>[2x]EKVDNPFEGAKLYVNPVWSAKAAAEPGGSAVANESTAVWLDRIGAIEGNDSPTTGSMGLRDHLEEAVRQSGGDPLTIQVVIYNLPGRDCAALASNGELGPDELDRYKSEYIDPIADIMWDFADYENLRIVAIIEIDSLPNLVTNVGGNGGTELCAYMKQNGGY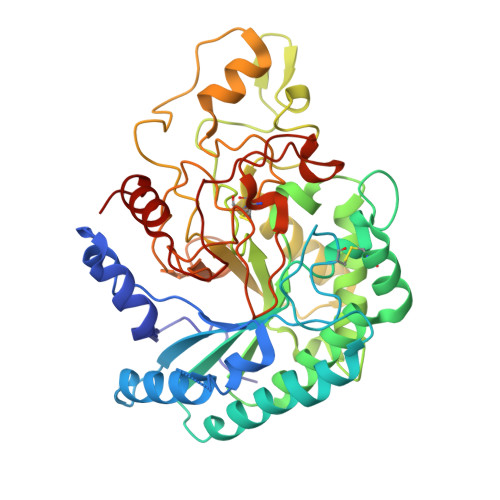VNGVGYALRKLGEIPNVYNYIDAAHHGWIGWDSNFGPSVDIFYEAANASGSTVDYVHGFISNTANYSATVEPYLDVNGTVNGQLIRQSKWVDWNQYVDELSFVQDLRQALIAKGFRSDIGMLIDTSRNGWGGPNRPTGPSSSTDLNTYVDESRIDRRIHPGNWCNQAGAGLGERPTVNPAPGVDAYVWVKPPGESDGASEEIPNDEGKGFDRMCDPTYQGNARNGNNPSGALPNAPISGHWFSAQFRELLANAYPPL3-(2-methoxyphenyl)-6-methyl[1,2]oxazolo[5,4-d]pyrimidin-4(5H)-one | C13 H11 N3 O3 | 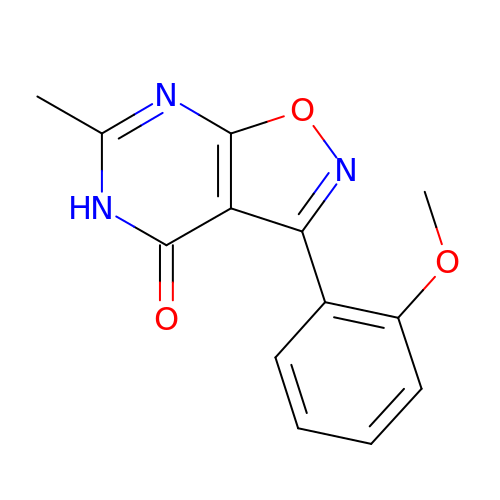XCLPDGVIHJQQOR-UHFFFAOYSA-N> ARSTNTFNYATYHTLDEIYD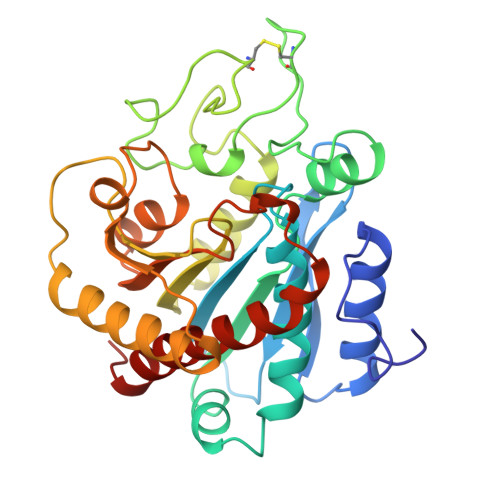FMDLLVAEHPQLVSKLQIGRSYEGRPIYVLKFSTGGSNRPAIWIDLGIHSREWITQATGVWFAKKFTEDYGQDPSFTAILDSMDIFLEIVTNPDGFAFTHSQNRLWRKTRSVTSSSLCVGVDANRNWDAGFGKAGASSSPCSETYHGKYANSEVEVKSIVDFVKDHGNFKAFLSIHSYSQLLLYPYGYTTQSIPDKTELNQVAKSAVEALKSLYGTSYKYGSIITTIYQASGGSIDWSYNQGIKYSFTFELRDTGRYGFLLPASQIIPTAQETWLGVLTIMEHTLNNLY> MGW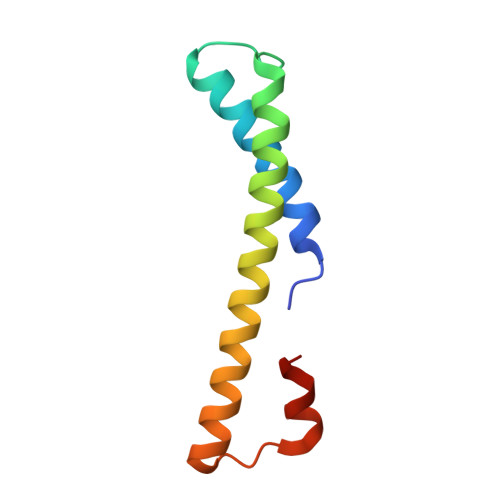EYAGTYGALCGMVYAIGSNVISGRAWFRRPWVHVTSVTLSYLGSKLLDEVQDTYYLEHLKRVERKGLQVTEEHKKLFSAY> GGCGUCGCUAGUA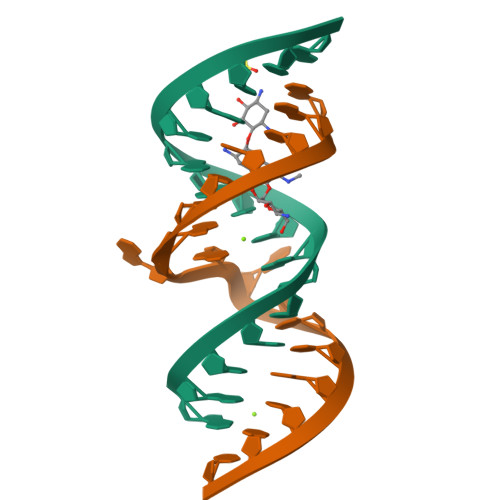CCG;> GGUACUAAAAGUCGCCC>[4x]MFQDNPLLAQLKQQLHSQTPRAEGVVKATEKGFGFLEVDAQK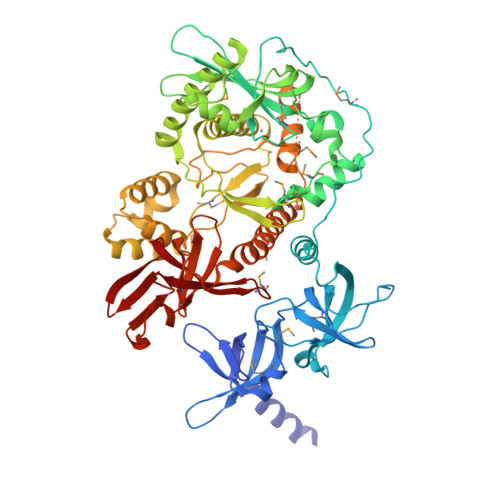SYFIPPPQMKKVMHGDRIIAVIHSEKERESAEPEELVEPFLTRFVGKVQGKNDRLAIVPDHPLLKDAIPCRAARGLNHEFKEGDWAVAEMRRHPLKGDRSFYAELTQYITFGDDHFVPWWVTLARHNLEKEAPDGVATEMLDEGLVREDLTALDFVTIDSASTEDMDDALFAKALPDDKLQLIVAIADPTAWIAEGSKLDKAAKIRAFTNYLPGFNIPMLPRELSDDLCSLRANEVRPVLACRMTLSADGTIEDNIEFFAATIESKAKLVYDQVSDWLENTGDWQPESEAIAEQVRLLAQICQRRGEWRHNHALVFKDRPDYRFILGEKGEVLDIVAEPRRIANRIVEEAMIAANICAARVLRDKLGFGIYNVHMGFDPANADALAALLKTHGLHVDAEEVLTLDGFCKLRRELDAQPTGFLDSRIRRFQSFAEISTEPGPHFGLGLEAYATWTSPIRKYGDMINHRLLKAVIKGETATRPQDEITVQMAERRRLNRMAERDVGDWLYARFLKDKAGTDTRFAAEIVDISRGGMRVRLVDNGAIAFIPAPFLHAVRDELVCSQENGTVQIKGETVYKVTDVIDVTIAEVRMETRSIIARPVA>[2x]KFAEHLSAHITPEWRKQYIQYEAFKDMLYSAQDQAPSVEVTDED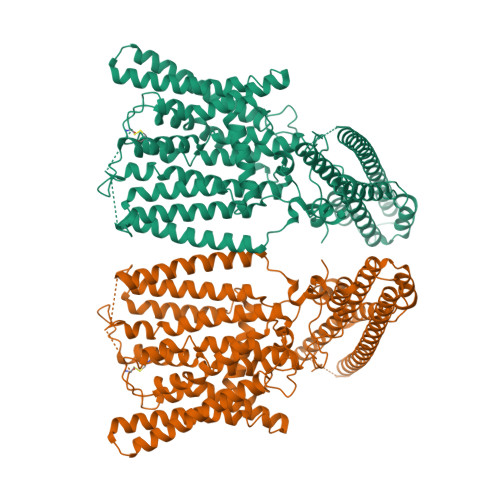TVKRYFAKFEEKFFQTCEKELAKINTFYSEKLAEAQRRFATLQNELQSSLDAQKESTGVTTLRQRRKPVFHLSHEERVQHRNIKDLKLAFSEFYLSLILLQNYQNLNFTGFRKILKKHDKILETSRGADWRVAHVEVAPFYTCKKINQLISETEAVVTNELEDGDRQKAMKRLRVPPLGAAQPAPAWTTFRVGLFCGIFIVLNITLVLAAVFKLETDRSIWPLIRIYRGGFLLIEFLFLLGINTYGWRQAGVNHVLIFELNPRSNLSHQHLFEIAGFLGILWCLSLLACFFAPISVIPTYVYPLALYGFMVFFLINPTKTFYYKSRFWLLKLLFRVFTAPFHKVGFADFWLADQLNSLSVILMDLEYMICFYSLELKWDESKGLLPNNSEESGICHKYTYGVRAIVQCIPAWLRFIQCLRRYRDTKRAFPHLVNAGKYSTTFFMVTFAALYSTHKERGHSDTMVFFYLWIVFYIISSCYTLIWDLKMDWGLFDKNAGENTFLREEIVYPQKAYYYCAIIEDVILRFAWTIQISITSTTLLPHSGDIIATVFAPLEVFRRFVWNFFRLENEHLNNCAEFRAVRDISVA>MTKTLPKDFIFGGATAAYQAEGATHTDGKGPVAWDKYLEDNYWYTAEPASDFYHKYPVDLELAEEYGVNGIRISIAWSRIFPTGYGEVNEKGVEFYHKLFAECHKRHVEPFVTLHHFDTPEALHSNGDFLNRENIEHFIDYAAFCFEEFPEVNYWTTFNEIGPIGDGQYLVGKFPPGIKYDLAKVFQSHHNMMVSHARAVKLYKDKGYKGEIGVVHALPTKYPYDPENPADVRAAELEDIIHNKFILDATYLGHYSDKTMEGVNHILAENGGELDLRDEDFQALDAAKDLNDF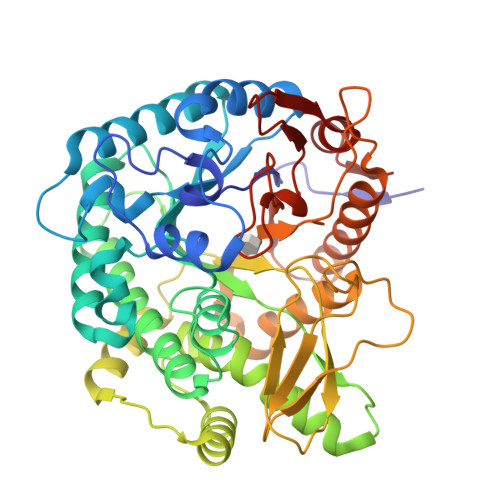LGINYYMSDWMQAFDGETEIIHNGKGEKGSSKYQIKGVGRRVAPDYVPRTDWDWIIYPEGLYDQIMRVKNDYPNYKKIYITCNGLGYKDEFVDNTVYDDGRIDYVKQHLEVLSDAIADGANVKGYFIWSLMDVFSWSNGYEKRYGLFYVDFDTQERYPKKSAHWYKKLAETQVIE[2x]> MPETRRSAGSDIPTPLVAVYADESCLGNGREGENPGGAGVLVEYARPGGAGDIVRRDVWVSEPATTNNRMALRSVIEAFRAIGHKGTRFRVVFTTDSRYIVDGMTRWVHDWAQRGWKRKSGA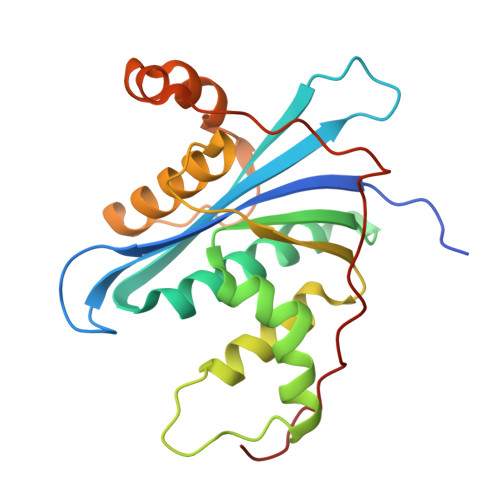IENLALWQEAVQAVNGHAVEWRWVRGHAGHAQNEYANHLAVTAAGGQTQSGGLVDSGYEEWAARVSTAASRMRLEPFPDAAAFRPSPALPVVAAGRPS N-(carboxymethyl)-N-(3-phenylpropyl)glycyl-N-methyl-L-histidinamide | C20 H27 N5 O4 | 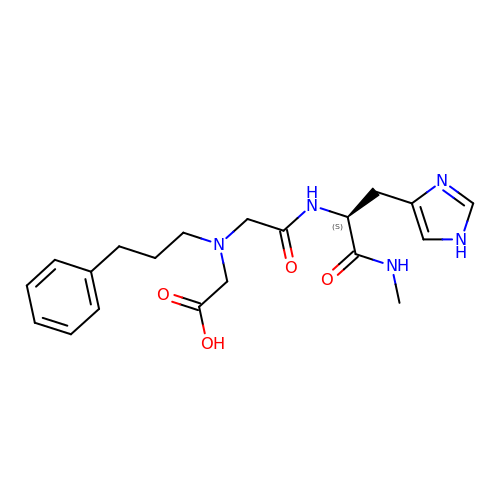QEPAXTJXHXPFJN-KRWDZBQOSA-N Picocyanobacteria strains encode a putative ABC-type phosphite/phosphate/phosphonate transporter, phnDCE, thought to provide access to an alternative phosphorus pool. To understand the function of the PhnDCE transport system and its ecological consequences, we characterised the PhnD1 binding proteins from four distinct marine Synechococcus isolates (CC9311, CC9605, MITS9220, and WH8102). We show the Synechococcus PhnD1 proteins selectively bind phosphorus compounds with a stronger affinity for phosphite than for phosphate or methyl phosphonate. However, based on our comprehensive ligand screening and growth experiments showing Synechococcus strains WH8102 and MITS9220 cannot utilise phosphite or methylphosphonate as a sole phosphorus source, we hypothesise that the picocyanobacterial PhnDCE transporter is a constitutively expressed, medium-affinity phosphate transporter, and the measured affinity of PhnD1 to phosphite or methyl phosphonate is fortuitous.

Therefore, to understand the molecular mechanism of Pi selectivity, we determined a high-resolution crystal structure (2.0 Å) of Synechococcus MITS9220_PhnD1 with bound Pi, resulting in a closed ligand-bound complex. The overall structure of MITS9220_PhnD1 is similar to that of other class II substrate binding proteins (SBPs) and specifically to cluster-F SBPs, with two α/β domains separated by a longer central hinge region (8–10 amino acids). The extended hinge region in cluster-F SBPs is believed to provide greater flexibility between the ligand-bound (closed) and unbound (open) conformations of cluster-F SBPs. This hinge region encompasses a buried ligand-binding cavity and includes a Pi molecule within the MITS9220_PhnD1 structure copurified with the protein. The MITS9220_PhnD1 structure displays an unusual asymmetric distribution of electrostatic surface potential, where the front is completely enveloped by positive charge, attracting several Cl- anions from the crystallisation buffer. Within the crystal structure of MITS9220_PhnD1, the four Pi oxygens are bound by a total of 10 direct hydrogen bonds, forming an extensive H-bond network to the main chain and sidechains of residues distributed between the two domains. These include a tyrosine (Y44) at the beginning of α2; an -STS- motif (S124, T125, S126) in a loop region joining β6 and α4; a histidine (H156) at the beginning of α6; an H-acceptor aspartic acid (D203) and a capping tyrosine residue (Y204) found just before β10. A single water molecule buried deep within the cavity also contributes to this hydrogen bond network. This water molecule is further stabilised by intramolecular hydrogen bonds to residues on domain 1 (T65) and domain 2 (S123), contributing to the interactions that connect the two domains and occluding the binding pocket from the solvent. Similarly, the capping Y204 sidechain is engaged in hydrogen bonds to residues D11 (domain 1) and N174 (domain 2), contributing to the two-domain interactions.

> GPMQPRLKVGAIPDQNPERLNRLYGQLADELSDRLNVKVRYVPVSNYPAAVSAFRTGGLDLVWFGGLTGVQARLQTPGAQVLAQRDIDARFRSVFIANTSSGLQPISSINGLTSLRGKRFSFGSESSTSGRLMPQHFLAKAGVTPSQFSGGRAGFSGSHDATIAVVQSGAYEAGALNEQVWTSAVNDGRVNTEKVSVIWRTPEYVDYHWVVRPKLDQRFGKGFTTRLQKAILGLEPTTPRQVTILELFAAKRFIPVEASQYKPIEKVGRELGKIR> MSGCTPKAAPAGATGRTTIAIDPVTRIEGHLKAEVVVENGKVVDARLSGGMYRGFETILRGRDPRDASQIVQRICGVCPTAHSTASVLALDEAFGAKVPNNGRITRNLIFGANYLQSHILHFYHLSAQDFVQGPDTAPFVPRFPKSDLRLSKELNK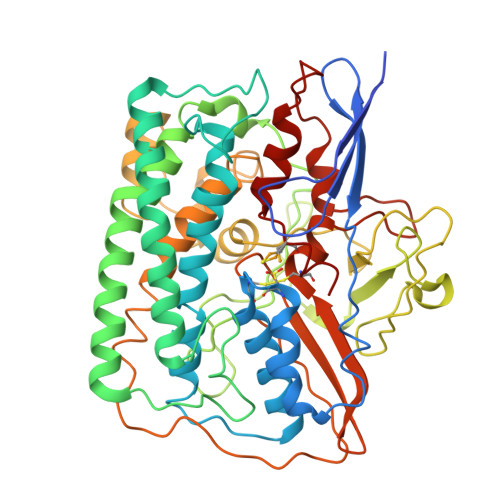AGVDQYIEALEVRRICHEMVALFGGRMPHVQGQVVGGATEIPTKEKLVEYAARFKKVRDFVEQKYVPVVYTIGSKYKDMFKVGQGFKAALCVGAFPLDNSGKKHLFMPGVYAKGKDMPFDPSKIKEYVKYSWFAEETTGLNYKEGKTIPAPDKAGAYSFVKAPRYDGLSLEVGPLARMWVNNPELSPVGKKLLKDLFGISAKKFRDLGEEAAFSLMGRHVARAEETYYMLGAIEGWLKEIKAGEDTVVMPAVPASAEGTGFTEAPRGSLLHYVKVKDSKIDNYQIVSASLWNCNPRDDMGQRGAVEEALIGIPVDDIQNPVNVARLIRAFDPULGCAVH>[8x]MTATAETSTGTKVVLGQNQYGKAEVRLVKVTRNTARHEIQDLNVTSQLRGDFEAAHTAGDNAHVVATDTQKNTVYAFARDGFATTEEFLLRLGKHFTEGFDWVTGGRWAAQQFFWDRINDHDHAFS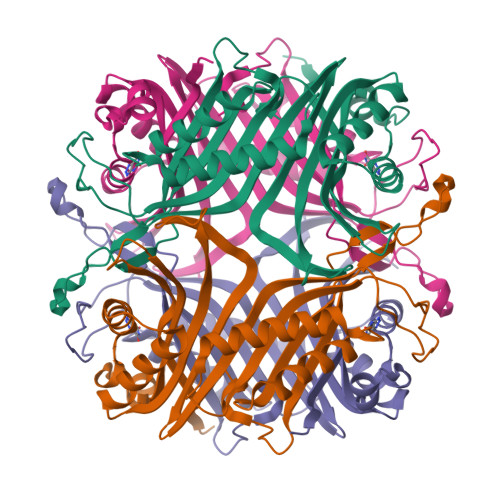RNKSEVRTAVLEISGSEQAIVAGIEGLTVLKSTGSEFHGFPRDKYTTLQETTDRILATDVSARWRYNTVEVDFDAVYASVRGLLLKAFAETHSLALQQTMYEMGRAVIETHPEIDEIKMSLPNKHHFLVDLQPFGQDNPNEVFYAADRPYGLIEATIQREGSRADHPIWSNIAGFC The two human DNA exonucleases containing an MBL-fold are SNM1A (also called DCLRE1A), a factor important for DNA interstrand cross-link (ICL) repair, and SNM1B (also called Apollo or DCLRE1B), a DNA repair factor that also plays an key role in maintaining overhangs at telomeres. The SNM1A and SNM1B/Apollo proteins are both classic 5′-3′ exonucleases, requiring a free 5′-phosphate to initiate digestion, but are members of a class of DNA processing factor family that have not previously been structurally characterized. The protein exhibits two structural domains: the metallo-β-lactamase (MBL) domain, arranged as a sandwich of two mixed β sheets (α/β-β/α); and the β-CASP domain, which is characteristic for a subset of MBL nucleases: CPSF-73, Artemis, SNM1A, Pso2, as well as RNaseJ. An extended active site in both enzymes includes, in addition to the canonical di-zinc catalytic centre, a binding pocket that defines the selectivity for terminal 5′ phosphate, and a wide binding groove which is essential for processivity and for the ability to digest past DNA damage sites.

A 2.16 Å crystal structure of SNM1B contains a single protein molecule in the asymmetric unit, with two coordinated zinc ions and two tartrate molecules at the active site. Motif 2, H31-X-H33-X-D35-H36, contributes two coordination bonds to each of the two zinc ions. H99 (motif 3) contributes the third bond to zinc-1, while a single oxygen of D120 (motif 4) bridges the two zinc ions. Zinc 1 is coordinated, in an octahedral arrangement, to the protein residues H31, H33, D120 and H99; two additional bonds are formed with the carboxyl (O4) and hydroxyl (O3) oxygens of a tartrate molecule (Tart_1) from the crystallization buffer. The shell around the second zinc is also octahedral, coordinated by the D35, H36, the bridging D120, the hydroxyl (O3) and second carboxyl (O1) oxygens of Tart_1, and one water molecule. The binding of tartrate_1 to the zinc centre is suggestive of a possible catalytic mechanism, whereby two oxygens of the phosphodiester to be cleaved are in positions similar to the tartrate carboxyl oxygens (O1 and O4), and a nucleophilic water or hydroxylate ion is coordinated to both zinc ions at the position of the tartrate O3 oxygen. Tartrate_2 is held in place by direct interactions with the side chains of Y182, K186, T257, S258, and S274, and the main chain amines of D275 and S258. The tight binding of tartrate may mimic binding of a 5′-terminal phosphate group of the DNA substrate. In SNM1B, D35 is held by a hydrogen bond to N2, which probably stabilizes the zinc-coordinating rotamer; there is no corresponding residue in SNM1A, and the amino-terminal is too distant in SNM1A to form such a contact.

> SMNGVLIPHTPIAVDFWSLRRAGTARLFFLSHMHSDHTVGLSSTWARPLYCSPITAHLLHRHLQVSKQWIQALEVGESHVLPLDEIGQETMTVTLLDANHCPGSVMFLFEGYFGTILYTGDFRYTPSMLKEPALTLGKQIHTLYLDNTNCNPALVLPSRQEAAHQIVQLIRKHPQHNIKIGLYSLGKESLLEQLALEFQTWVVLSPRRLELVQLLGLADVFTVEEKAGRIHAVDHMEICHSNMLRWNQTHPTIAILPTSRKIHSSHPDIHVIPYSDHSSYSELRAFVAALKPCQVVPIVSRRPCGGFQDSLSPRISVPLIPDSVQQYMSSFSRKPS>[2x]TPPPTQWSYLCHPRVKEVQDEVDGYFLENWKFPSFKAVRTFLDAKFSEVTCLYFPLALDDRIHFACRLLTVLFLIDDVLEHMSFADGEAYNNRLIPISRGDVLPDRTKPEEFILYDLWESMRAHDAELANEVLEPTFVFMRAQTDRARLSIHELGHYLEYREKDVGKALL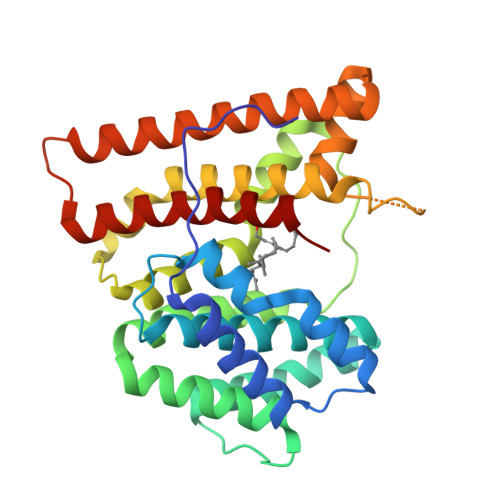SALMRFSMGLRLSADELQDMKALEANCAKQLSVVNDIYSYDKEEEASRTGHKEGAFLCSAVKVLAEESKLGIPATKRVLWSMTREWETVHDEIVAEKIASPDGCSEAAKAYMKGLEYQMSGNEQWSKTTR> PISPIETVPVKLKPGMDGPKVKQWPLTEEKIKALVEICTEMEKEGKISKIGPENPYNTPVFAIKKKDSTKWRKLVDFRELNKRTQDFWEVQLGIPHPAGLKKKKSVTVLDVGDAYFSVPLDEDFRKYTAFTIPSINNETPGIRYQYNVLPQGWKGSPAIFQSSMTKILEPFRKQNPDIVIYQYMDDLYVGSDLEIGQHRTKIEE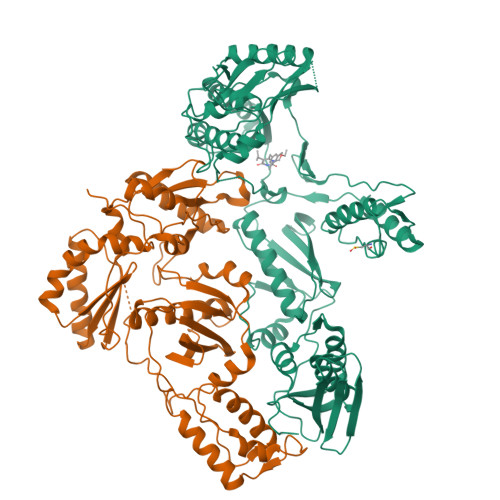LRQHLLRWGLTTPDKKHQKEPPFLWMGYELHPDKWTVQPIVLPEKDSWTVNDIQKLVGKLNWASQIYPGIKVRQLCKLLRGTKALTEVIPLTEEAELELAENREILKEPVHGVYYDPSKDLIAEIQKQGQGQWTYQIYQEPFKNLKTGKYARMRGAHTNDVKQLTEAVQKITTESIVIWGKTPKFKLPIQKETWETWWTEYWQATWIPEWEFVNTPPLVKLWYQLEKEPIVGAETFYVDGAANRETKLGKAGYVTNRGRQKVVTLTDTTNQKTELQAIYLALQDSGLEVNIVTDSQYALGIIQAQPDQSESELVNQIIEQLIKKEKVYLAWVPAHKGIGGNEQVDKLVSAGIRKVL;> PISPIETVPVKLKPGMDGPKVKQWPLTEEKIKALVEICTEMEKEGKISKIGPENPYNTPVFAIKKKDSTKWRKLVDFRELNKRTQDFWEVQLGIPHPAGLKKKKSVTVLDVGDAYFSVPLDEDFRKYTAFTIPSINNETPGIRYQYNVLPQGWKGSPAIFQSSMTKILEPFKKQNPDIVIYQYMDDLYVGSDLEIGQHRTKIEELRQHLLRWGLTTPDKKHQKEPPFLWMGYELHPDKWTVQPIVLPEKDSWTVNDIQKLVGKLNWASQIYPGIKVRQLCKLLRGTKALTEVIPLTEEAELELAENREILKEPVHGVYYDPSKDLIAEIQKQGQGQWTYQIYQEPFKNLKTGKYARMRGAHTNDVKQLTEAVQKITTESIVIWGKTPKFKLPIQKETWETWWTEYWQATWIPEWEFVNTPPLVKLWYNLEKEPIVGAETF During the late phase of HIV-1 infection, viral Gag polyproteins are targeted to the plasma membrane (PM) for assembly. Gag localization at the PM is a prerequisite for the incorporation of the envelope protein (Env) into budding particles. Gag assembly and Env incorporation are mediated by the N-terminal myristoylated matrix (MA) domain of Gag. Pioneering X-ray crystallography studies of HIV-1 unmyristoylated MA [myr(–)MA] revealed that the protein adopts a trimer arrangement.

When mapped on the putative hexamer of trimer model of MA, these residues were found to point toward the hexamer centers. It was also shown that substitution of residue Gln63 with Arg suppressed Env incorporation defects of the L13E, E17K, L31E, V35E, or E99V MA mutations and of a gp41CT mutation that has the same phenotype. To explain the role of MA trimerization in Env incorporation, it was suggested that the Q63R mutation in MA may stabilize the trimer structure such that MA lattices that form large hexamer holes are favored over those that feature small hexamer holes. However, it is not clear how this substitution can stabilize the trimer form. To be able to assess the structural changes in the MA trimer, we determined the high-resolution structure of myr(–)MA Q63R protein by X-ray crystallography. Interestingly, the two crystal forms of myr(–)MA Q63R yielded structures that are essentially identical with slightly different parameters. Each asymmetric unit of the crystal structure contains two trimers. The structure of the myr(–)MA Q63R trimer in both crystal forms is virtually identical to that of the WT myr(–)MA protein with slight orientation differences of monomers in the trimeric assembly. The structures in the two crystal forms revealed only minor conformational changes in the loops connecting helices I and II and helices V and VI. Intriguingly, the guanidinium group of Arg63 is 2.5 Å (averaged across 12 examples in the asymmetric unit of the two crystal forms) from the hydroxyl group of Ser67 of an adjacent MA molecule, which forms new hydrogen bonding in the trimer interface. Our findings complemented the biological data by showing that the H-bond formed between the side chains of Arg63 and Ser67 is key for the stability of the MA trimer and hence to its function in rescuing Env incorporation.

>GARASVLSGGELDKWEKIRLRPGGKKQYKLKHIVWASRELERFAVNPGLLETSEGCRQILGRLQPSLQTGSEELRSLYNTIAVLYCVHQRIDVKDTKEALDKIEEEQNKSKKKAQQAAADTGNNSQVSQNYHHHHHH[6x]> AQEEEAEQNLSELSGPWRTVYIGSTNPEKIQENGPFRTYFRELVFDDEKGTVDFYFSVKRDGKCKNVHVKAT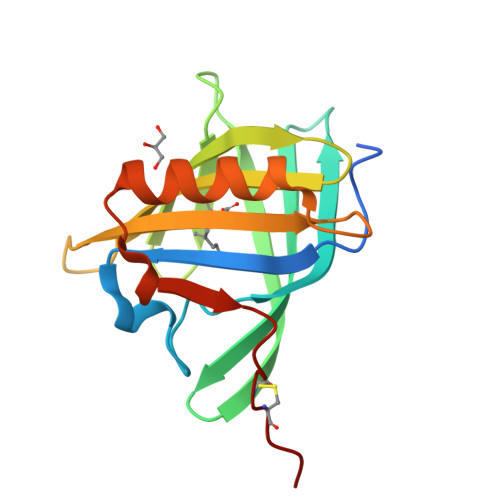KQDDGTYVADYEGQNVFKIVSLSRTHLVAHNINVDKHGQTTELTELFVKGLNVEDEDLEKFWKLTEDKGIDKKNVVNFLENEDCPHPE>GPHMLEAEHPLQYNYTFWYSRRTPGRPTSSQSYEQNIKQIGTFASVEQFWRFYSHMVRPGDLTGHSDFHLFKEGIKPMWEDDANKNGGKWIIRLRKGLASRCWENLILAMLGEQFMVGEEICGAVVSVRFQEDIISIWNKTASDQATTA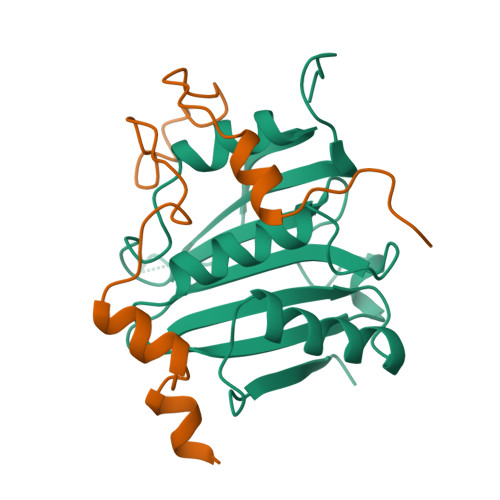RIRDTLRRVLNLPPNTIMEYKTHTDSIKMPGRLGPQRLLF[2x];>GPHMKYKLADYRYGREEMLALFLKDNKIPSDLLDKEFLPILQEEPLPPLALVPFTEEEQRNFSMSVNSAAVLRLT[2x]> HVFIRTELSFIKNNVPCIRDMFFIYKRELYNICLDDLKGEEDETHIYVQKKVKDSWITLNDLFKETDLTGRPHIFAYVDVEEIIILLCEDEEFSNRKKDMTCHRFYSNDGKEYQNSEIT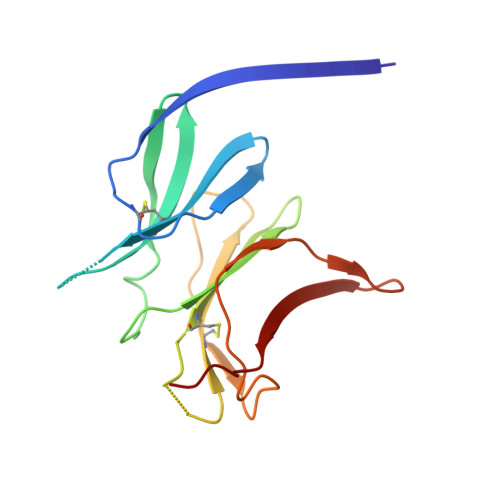ISDYILKDKLLSSYVSLPLKIENREYFLICGVSPYKFK>[2x]SNAAPAPAPAPEVQTKHFTLKSDVLFNFNKSTLKPEGQQALDQLYSQLSNLDPKDGSVVVLGFTDRIGSDAYNQGLSEKRAQSVVDYLISKGIPSDKISARGMGESNPVTGNT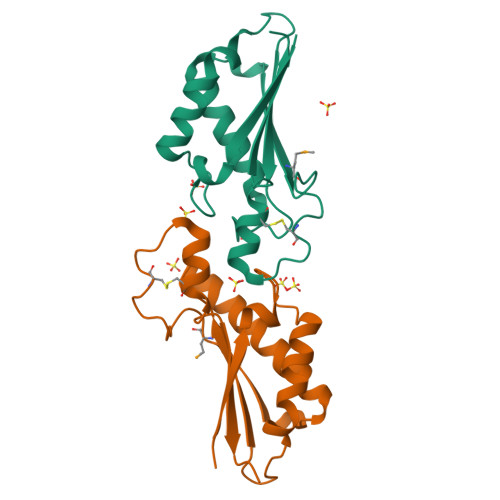CDNVKPRAALIDCLAPDRRVEIEVKGVKDVVTQPQ Fetuin-B is a highly selective and potent inhibitor of metallo­peptidases (MPs) of the astacin family, which includes ovastacin in mammals. By inhibiting ovastacin, fetuin-B is essential for female fertility. The crystal structure of fetuin-B was determined unbound and in complex with archetypal astacin, and it was found that the inhibitor has tandem cystatin-type modules (CY1 and CY2). They are connected by an exposed linker with a rigid, disulfide-linked ‘CPDCP-trunk’, and are followed by a C-terminal region (CTR) with little regular secondary structure.

Examination of the crystal packing of the protein expressed in mammalian cells explains why it crystallized in its unbound form, whereas the material produced in insect cells did not: endoglycosidase H processing of the high-mannose N-glycans of the HEK293S-derived protein (a step performed during purification) left a single N-acetyl­glucosamine moiety attached to N40 that stacks against W200 of a symmetry-related molecule. This introduces a crucial crystal-packing contact that would most likely be hindered by the presence of additional sugar residues attached to the core N-acetylglucosamine, such as those normally found in proteins expressed in insect cells. The respective cores comprising CY1+LNK+CY2 are undefined for both the tip of hairpin II and Lβ8β9 of CY2, and they superpose with an r.m.s.d. of 1.7 Å. CY1 and CY2 are just rotated by ∼10° with respect to each other when going from the unbound to the complexed structure. The only functionally relevant differences in the cores are found at the tips of hairpins I and II of CY2 [inset in Fig. 1(e)], which however are very likely to result from crystal contacts in the unbound structure. Hairpin I is in a noncompetent conformation for binding, and becomes folded out towards the CPDCP-trunk upon complex formation.

> RSPPAPPLPQRPLSPLHPLGCNDSEVLAVAGFALQNINRDQKDGYMLSLNRVHDVREHYQEDMGSLFYLTLDVLETDCHVLSRKAQKDCKPRMFYESVYGQCKAMFHINKPRRVLYLPAYNCTLRPVSKRKTHTTCPDCPSPIDLSNPSALEAATESLAKFNSKSPSKKYELVKVTKAMNQWVSGPAYYVEYLIKEAPCTKSQASCSLQHSDSEPVGICQGSTVQSSLRHVPLIQPVEKSVTVTCEFFESQAQVPGDENPAVTQGPQKLPQKNTAPTSSPSVTAPRGSIQHLPELDDEKPEESKGGSPEEAFPVQLDLTTNPQGDTLDVSFLYLEPGDKKLVVLPFPGKEQRSAECPGPEKENNPLVLPPLEHHHHHH THYMINE | C5 H6 N2 O2 | 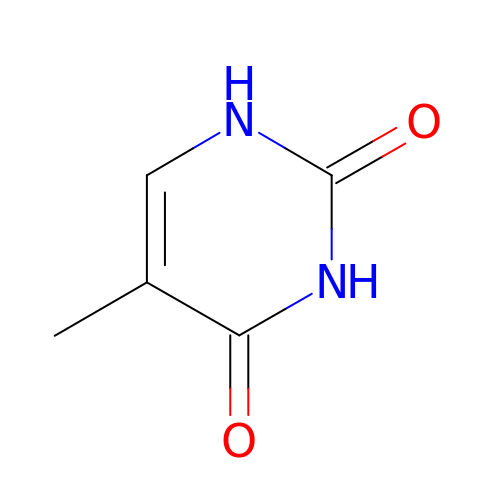RWQNBRDOKXIBIV-UHFFFAOYSA-N> DDYLDRLPKSKKGLQGLLQDIEKRILHYKQLFFKEQNEIANGKRSMVPDNSIPICSDVTKLNFQALIDAQMRHAGKMFDVIMMDPPWQLSSSQPSRGVAIAYDSLSDEKIQNMPIQSLQQDGFIFVWAINAKYRVTIKMIENWGYKLVDEITWVKKTVNGKIAKGHGFYLQHAKESCLIGVKGDVDNGRFKKNIASDVI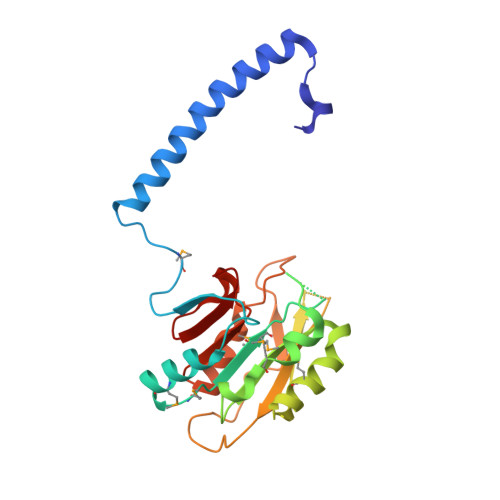FSERRGQSQKPEEIYQYINQLCPNGNYLEIFARRNNLHDNWVSIGNEL>[2x]UUG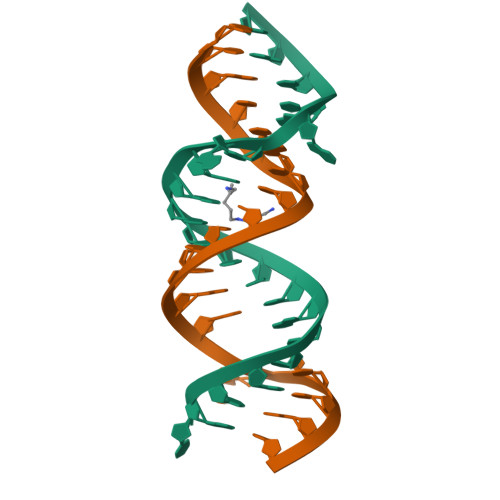CGUCGCUCCGGAAAAGUCGC>[3x]MDTNQKLSIAVFALGCFWGPDAQFGSIKGVVSTRVGYAGGTTNNPSYYNLGDHSESIEIQYDANVITYGELLNIFWNLHNPVYETTNRQYMSRIFYLDDGQKSEALEMKRQIEAANGEKIY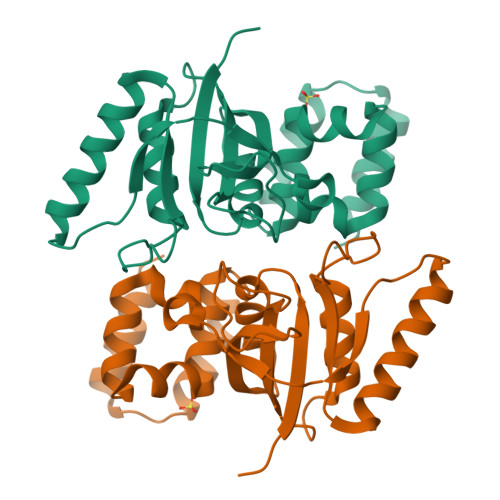TEIVPLENFYLAEGYHQKYYLQNTTKLYQTLKAIYGGFGNLVRSTLAARMNGYIAGNLSIASLKEEMDLVELPEDQYEKVLSIVEEIK>GAHMDCHLSDMLQQLHSVNASKPSERGLVRQEEAEDPACIPIFWVSKWVDYSDKYGLGYQLCDNSVGVLFNDSTRLILYNDGDSLQYIERDGTESYLTVSSHPNSLMKKITLLKYFRNYMSEHLLKAG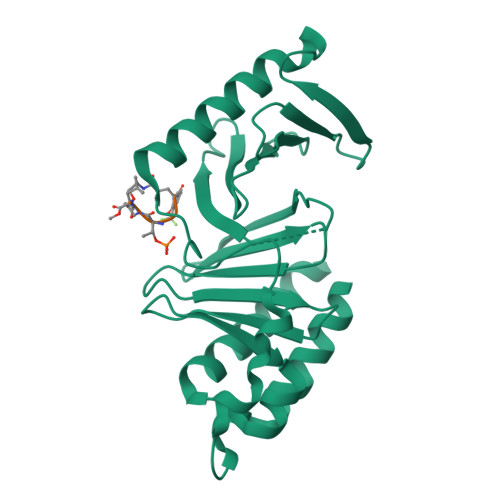ANITPREGDELARLPYLRTWFRTRSAIILHLSNGSVQINFFQDHTKLILCPLMAAVTYIDEKRDFRTYRLSLLEEYGCCKELASRLRYARTMVDKLLSSRSASNRLKAS[2x]> MGNYFESPFRGKLLSEQVSNPNIRVGRYSYYSGYYHGHSFDDCARYLMPDRDDVDKLVIGSFCSIGSGAAFIMAGNQGHRAEWASTFPFHFMHEEPAFAGAVNGYQPAGDTL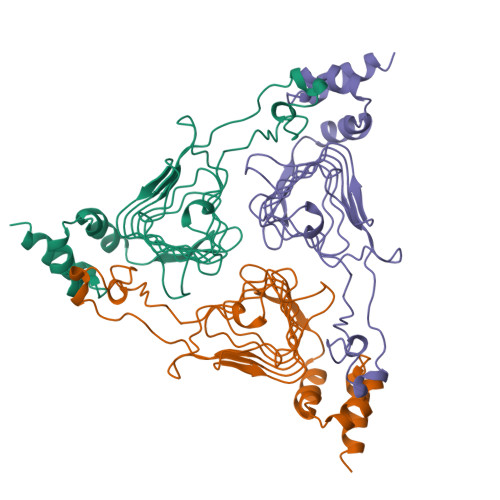IGHEVWIGTEAMFMPGVRVGHGAIIGSRALVTGDVEPYAIVGGNPARTIRKRFSDGDIQNLLEMAWWDWPLADIEAAMPLLCTGDIPALYQHWKQRQATA>ACUCGUUUGAGCGAGUAUAAACAGCUGGUUAAGCUCAAAGCGGAGAGCAGA[2x];>UCUGCUCUCX[2x];>[2x]UCCAG

Small self‐cleaving ribozymes catalyze site‐specific cleavage of their own phosphodiester backbone. They are widely distributed in nature and are essential for rolling‐circle‐based replication of satellite and pathogenic RNAs. Comparative genomic analysis led to the discovery of novel self‐cleaving ribozymes, named twister, twister‐sister, pistol, and hatchet. In the present study we set out to obtain conformational snapshots along the reaction coordinate of the pistol ribozyme phosphordiester cleavage. We succeeded in solving the X‐ray structures of both its TS analogue vanadate (at 2.8 Å resolution) and the ternary 2′,3′ cyclophosphate product complex (at 2.65 Å resolution; see Figure S1 in the Suppporting Information for stereoviews).

The third structural snapshot on the pistol ribozyme reaction coordinate that we have solved represents the post‐cleavage state. In this product structure, G53 and U54 are slightly more distant to each other compared to the TS analogue. Moreover, the ribose moiety of G53 finds itself in a distinctly different orientation, with its 2′,3′‐cyclic phosphate rotated relative to the vanadate moiety in the TS mimic. As a result, the cyclic phosphate is recognized by a 2.6 Å hydrogen bond between G40‐N1 and its pro‐S nonbridging oxygen atom, and a 3.0 Å hydrogen bond between the free 5′OH and its nonbridging pro‐R oxygen atom. Notably, the divalent metal ion remains coordinated to the N7 of G33 (2.3 Å) and its 2.8 Å distance to the pro‐R oxygen of the cyclic phosphate offers the possibility for a water‐mediated interaction. Importantly, the structure of the pistol product complex clearly shows a second metal ion that was located at a 4.0 Å distance to the pro‐S oxygen atom of the cyclic phosphate, and therefore also offers the possibility for outershell, water‐mediated hydrogen bonding. In the product structure, G42 is redirected towards G40 (2.8 Å distance between G42‐O6 and G40‐N2). Simultaneously, the cyclophosphate terminus of G53 slides away, with its N2 in over 4.4 Å distance to O6‐G42. The resulting cyclic phosphate product is embedded in a narrowed hydrogen‐bond network involving two divalent ions (Mg2+) in outersphere coordination to pro‐R and pro‐S oxygen centers, respectively. This arrangement may contribute to the stabilization of a cyclophosphate conformation that prevents ligation of the cleaved fragments (reversible reaction).>GSHMPPNRPGITFEIGARLEALDYLQKWYPSRIEKIDYEEGKMLVHFERWSHRYDEWIYWDSNRLRPLER[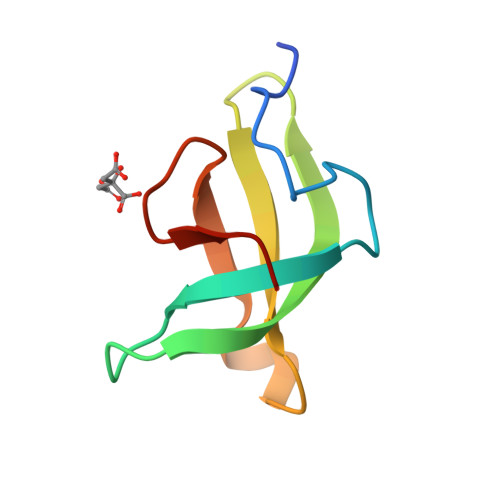2x]>[2x]MPI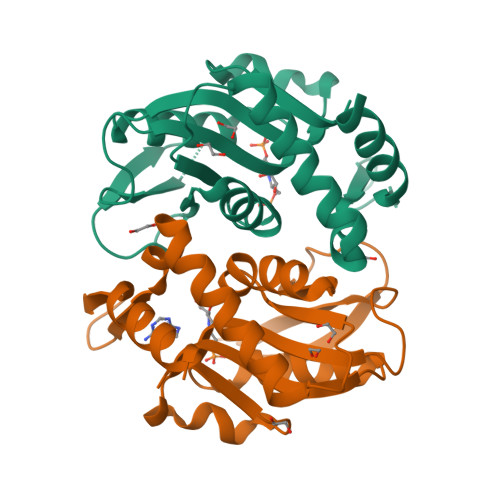ASYAQELKLALHQYPNFPSEGILFEDFLPIFRNPGLFQKLIDAFKLHLEEAFPEVKIDYIVGLESRGFLFGPTLALALGVGFVPVRKAGKLPGECFKATYEKEYGSDLFEIQKNAIPAGSNVIIVDDIIATGGSAAAAGELVEQLEANLLEYNFVMELDFLKGRSKLNAPVFTLLNAQKEALKK Mitochondrial ATP synthase consists of the soluble F1 and membrane-bound Fo subcomplexes and occurs in dimers that assemble into oligomers to induce the formation of inner-membrane folds, called cristae. Dissociation of ATP synthase dimers into monomers results in the loss of native cristae architecture and impairs mitochondrial function. Here, we report cryo-EM structures of the intact ATP synthase dimer from Trypanosoma brucei in ten different rotational states. Although overall dimer architecture varies among eukaryotes, we find that subunit-g together with subunit-e form an ancestral oligomerization motif, which is shared between the trypanosomal and mammalian lineages.

Using masked refinements, maps were obtained for the membrane region, the rotor, and the peripheral stalk. The membrane region includes eight conserved Fo subunits (b, d, f, 8, i/j, k, e, and g) arranged around the central proton translocator subunit-a. For subunit-b, a single transmembrane helix superimposes well with bH1 from yeast and anchors the subunits-e and -g to the Fo. In our structure, the lumenal half-channel, which displays a local resolution of 2.55 Å, is filled with a network of resolved water densities, ending in a chain of five ordered water molecules (W1–W5). The presence of ordered water molecules in the aqueous channel is consistent with a Grotthuss-type mechanism for proton transfer, which would not require long-distance diffusion of water molecules. The distance of 7 Å between the last resolved water (W1) and D202a, the conserved residue that is thought to transfer protons to the c-ring, is too long for direct proton transfer. Instead, it may occur via the adjacent H155a. Instead, the position of bH2 is occupied by a fully ordered phosphatidylcholine in our structure (PC1). The e/g module is held together by four bound cardiolipins in the matrix leaflet, anchoring it to the remaining Fo region.

>MFLFFFCDLFWLRLLLCMYYCVWSRLCFIVYFNCLMLIFDFLLFCLFDLYLFVGLCLFLLLWFMLFNLYSLILYYCITYLNLYLLFCIVFLLYIAFLFLFCFLCDFFLFNNLLVGDSFMDVFFIRFLLCFLECFSLLCRCLSTFLRLFCNLLSSHFLLLMFFDFFYFIFVFFFYGVFCYWFILFIFVFCFCLLFYVFLYLLDLFAAILQLFIFCNMILQLIMDFLLFLLFV[2x];>[2x]MLRRLGANVSNMARPMNKYAVTVSPRRHLEPMSTWYLASWAMVWYYAFFFWMPMVWTDIMVPSFVYNKLPVIHFLQEKRAEQKLRRVLDETYTEWTEELDQAHVTDAITRSLNI;>MRRVSSPNITIQSVRWISGVSPLLYFPPTTTSTTNREDQINKNTNIAIQMIKRYKGEVPPHYTRKSSATIEQVEKEIDALLGGAEKLRKTSTDDQPMDKLTLMERCLRHALWSYHKEEGRYDFDQIGRWVVYTPEDEVKLAQLKREVEAKEKLAALRKRREEEGLPGGPVPRINWPQEYSSFIDREPVVAKRIRYDTLASTTLERDEKQIESTLQQYRRASQDKRLDDLVDLLERFKPVLAREAIMQRLTIKHLEGQLGVWRYMDWCPEVRDRAELEVDITGWQWWSPLEERRLLPVRLRSVNEVREIMSKTQAKKSAEAAERNPIVTQTSTGDNARDRLLKEVLALQARINQRDEVEPSQTEQKKKAHH[2x];>MQGSWSVLKKNCSNFFPGLLAFAQQTQEAYGIWLRIYNRQQKYGPTDFVEQSETFSPDYHKRFHSQDKNMWVDKELCTEVSQKEVARLMTYKLDMWRMAHCAGALLATGGYAIPFGLFWLANDTWVPSSFNLTGEELRAWREAQDLYRYRSAPSYLTDTKWHFDFHAYPWNETQERAWDDLFEKNDVRRDPKVVRPAAEMYDGFIKFELIRRKSLRHLCRSMNIPTFPMLARLCNGTRVRDYWNLAWCEDYMVITQRLHESMTDEELYDYAWRRYLAPYDKNLNREQLMERVEDYFEFLGPDFVAHGKAPNLVILTNYVLGYYNDPAYLEGDISELDKNDYDHLASWGKDAFLRRLEFENGPLRDQVEAHTQRLLAERAAIAKGDNAAAVEGRHTA[2x];>MVLFSTYRSSRLVSKEFLHGPVMRFRALGEYYFQRAWNGTLNWALPGEYRLYAVMIPFIYFYHRWHNDHTLDRDHVEKAMIMRWGGTLEDVRKLSAKDQLRVRCFTDIEKLYSAYGPKDTYLQPPGDTLPGKDFYRKAGGAQAHH[2x];>[2x]MVYTRWKCDRLPVFQLKLFTQEYPMHAAVGIFTIIFLWKHMSHCSEETERKYGWWAGYPYWRDPIARRNETKYKQMIINNDVDITHPKWTGCSVEQLEELSRVV;>MTKYELKMQYFDEWMIRWRKFQTESDWEIEKGRQWWRRFNMAVSGALFCGLVLYTSGTATLKRQYGLPHFFDIGVDGQAKETMLKTLTSRWRYTPQGYGRVLITGVPTYILFVTLEHYRERRRMQQYLQQNTVFGEQMRRLLSTGKIEEYLPVNIKATLPASQQAIYNY[2x];>MLRRSSAALIRRTPVRHSGGELFVRPKLEEIPPADQCRGFFGPLNDSLKFLRLLDIKWMMNRAVAMRREYLIATPTLFTFIWMFTWKGAVIYFWGDRAPPRRMDWNTEETGRLPLGFKPTPAPL[2x];>[2x]MSAKAAPKTLHQVRNVAYFFAAWLGVQKGYIEKSANDRLWVEHQRKVRQQNVERQQALDSIKLMQQGVRATTPGQLEGVPAELQQLAEAFTK;>[2x]MSSTKCAVACKIMTPLCNAASKVQARSAKKLAALTDAGIQKTISEHNANGTDAAVSSTKRYLAEQRQLFHYRVVRFFDECHYIISGEYFAQYTKVNLIWDLRFLTKLVVLFLIGTVLGRQSIFPPIDPDSPLVEALVTKVNPNY;>[2x]MLRKTPLFAMATTRKALVGNGPTFSTGGECMNTCDIQNAFPMNDRGVRSSSPFQEPNTAIYDSYLAWTYFQPMDVHIEKLPAPEAKYYQRHTKKPWDVSSTELTEIQSRKKYFQTLGYLVAFIYLYFLMPKEKSFSGLSGPDGHWIMLPKGRPELF;>MSSGFHFHDVSNDAIKGMPPSEALHKHLENAQLAHRICLAKALKAGEPPVEKCALTWGEVLIRYQAWSEYRPPFQDSVAQAKYKKYWSKKRQEEDDKNPFK[2x];>MLRRLVPRVMMAPMGGATALCTSRGYNMLVFRDPKRRPQLSEEERAKVVVNQAEWPEEFKDFDPDDPYKNSPEIIKGMSSWNLFLWGVECAFIYQFYELVFPKSI[2x];>[2x]MTENIEAVMSDFWSNPADHFRPNLKALTLYAERQHYVDRWLHVKERWLAPWYLPWWSPLFQLGTWYSQRSRNLFLVENHLSYRPYKFRRNDEDRNNPY;>MLLGGFVPRRFSQFNRDPCWMFFIFSVGFWLGEYPAMMIKYNARDLVYDPHRYVWSHHDDHH[2x]> MSADAQSFLNRVCGVSAARLTPCGTGTSTDVVYRAFDIYNDKVAGFAKFLKTNCCRFQEKDEDDNLIDSYFVVKRHTFSNYQHEETIYNLLKDCPAVAKHDFFKFRIDGDMVPHISRQRLTKYTMADLVYALRHFDEGNCDTLKEILVTYNCCDDDYFNKKDWYDFVENPDILRVYANLGERVRQALLKTVQFCDAMRNAGIVGVLTLDNQDLNGNWYDFGDFIQTTPGSGVPVVDSYYSLLMPILTLTRALTAESHVDTDLTKPYIKWDLLKYDFTEERLKLFDRYFKYWDQTYHPNCVNCLDDRCILHCANFNVLFSTVFPPTSFGPLVRKIFVDGVPFVVSTGYHFRELGVVHNQDVNLHSSRLSFKELLVYAADPAMHAASGNLLLDKRTTCFSVAALTNNVAFQ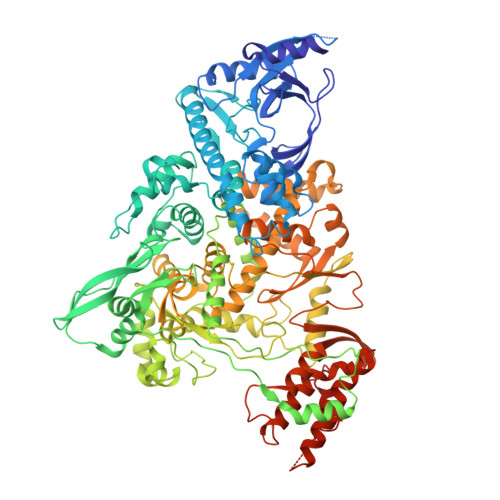TVKPGNFNKDFYDFAVSKGFFKEGSSVELKHFFFAQDGNAAISDYDYYRYNLPTMCDIRQLLFVVEVVDKYFDCYDGGCINANQVIVNNLDKSAGFPFNKWGKARLYYDSMSYEDQDALFAYTKRNVIPTITQMNLKYAISAKNRARTVAGVSICSTMTNRQFHQKLLKSIAATRGATVVIGTSKFYGGWHNMLKTVYSDVENPHLMGWDYPKCDRAMPNMLRIMASLVLARKHTTCCSLSHRFYRLANECAQVLSEMVMCGGSLYVKPGGTSSGDATTAYANSVFNICQAVTANVNALLSTDGNKIADKYVRNLQHRLYECLYRNRDVDTDFVNEFYAYLRKHFSMMILSDDAVVCFNSTYASQGLVASIKNFKSVLYYQNNVFMSEAKCWTETDLTKGPHEFCSQHTMLVKQGDDYVYLPYPDPSRILGAGCFVDDIVKTDGTLMIERFVSLAIDAYPLTKHPNQEYADVFHLYLQYIRKLHDELTGHMLDMYSVMLTNDNTSRYWEPEFYEAMYTPHTVLQGGSENLYFQG> LSAQ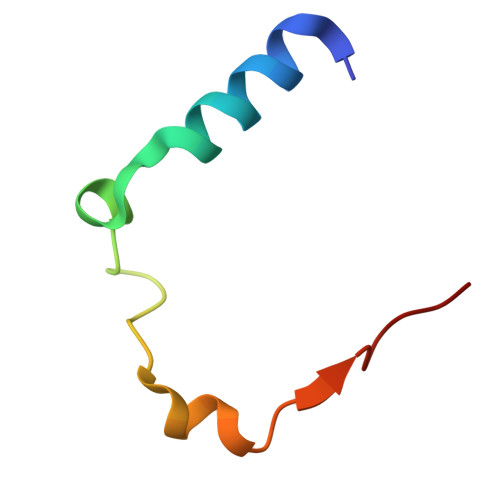HEAELKALAKKSDDEIDYSDIPASEDGQWSEAVRGKFFRP> MQFIDVEFPRDIAAGCQAVLTRRDEVVTLASGREEVNSRWADTRRSWDAGLGVRDEADLAQVVALFEEVRGRLYAFRFRDWLDWRTAATRAPITATDQPLGLGDGSRTAFQVVKVYGAVNPYTRPL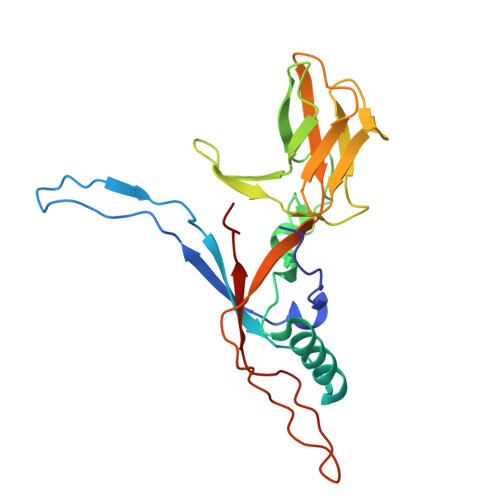SLPHPGTVRVALDGVTQPSGWTLTAPGGVITFDTPPALGVTVTAGCSFDVPVRFSDPELAVQWAYFREGQAGLAQAPSIPLIEVRLDP>[4x]GPLGSSKYNFQTAPNRLSHHTYKWKETETDPQLLPAWIADMDFEVMPEVKQAIHDYAEQLVYGYTYASDELLQAVLDWEKSEHQYSFDKEDIVFVEGVVPAISIAIQAFTKEGEAVLINSPVYPPFA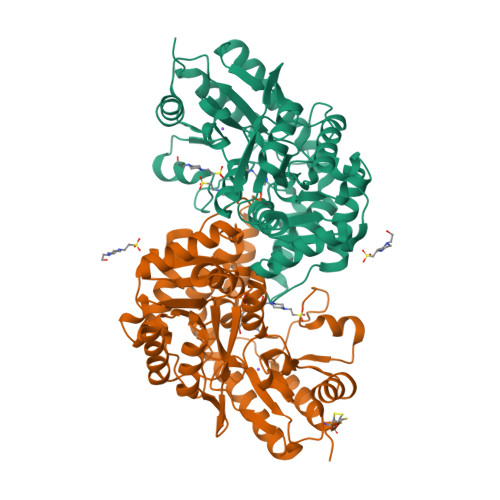RSVRLNNRKLVSNSLKEENGLFQIDFEQLENDIVENDVKLYLLCNPHNPGGRVWEREVLEQIGHLCQKHHVILVSDEIHQDLTLFGHEHVSFNTVSPDFKDFALVLSSATKTFNIAGTKNSYAIIENPTLCAQFKHQQLVNNHHEVSSLGYIATETAYRYGKPWLVALKAVLEENIQFAVEYFAQEAPRLKVMKPQGTYLIWLDFSDYGLTDDALFTLLHDQAKVILNRGSDYGSEGELHARLNIAAPKSLVEEICKRIVCCLPK> KRAALIQNLRDSYTETSSFAVIEEWAAGTLQEIEGIAKAAAEAHGVIRNSTYGRAQAEKSPEQLLGVLQRYQDLCHNVYCQAETIRTVIAIRIPEHKEADNLGVAVQHAVLKIIDELEIKTLGSGEKSGSGGAPTPIGMYALREYLSARSTVEDKLLGSVDAESGKTKGGSQSPSLLLELRQIDADFMLKVELATTHLSTMV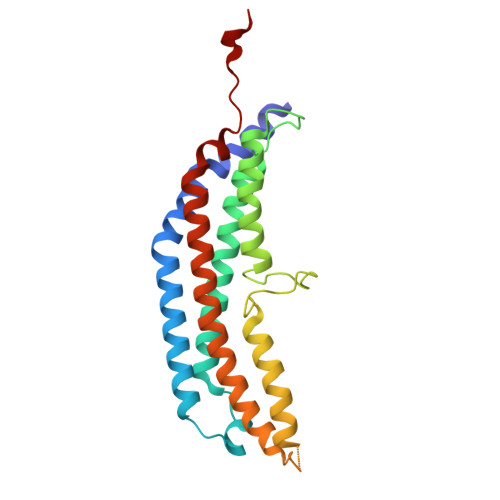RAVINAYLLNWKKLIQPRTGTDHMYS>[2x]SETSRTAFGGRRAVPPNNSNAAEDDLPTVELQGVVPRGVNLQEFLNVTSVHLFKERWDTNKVDHHTDKYENNKLIVRRGQSFYVQIDFSRPYDPRRDLFRVEYVIGRYPQENKGTYIPVPIVSELQSGKWGAKIVMREDRSVRLSIQSSPKCIVGKFRMYVAV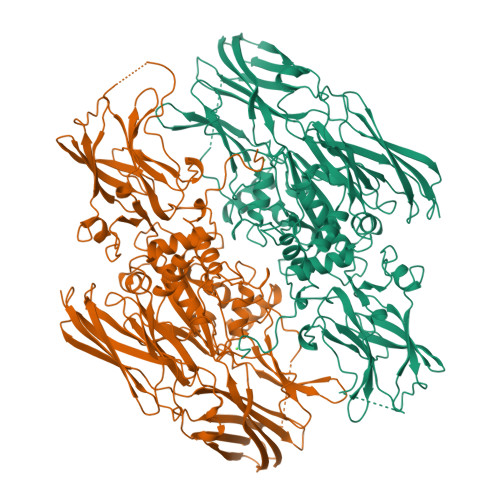WTPYGVLRTSRNPETDTYILFNPWCEDDAVYLDNEKEREEYVLNDIGVIFYGEVNDIKTRSWSYGQFEDGILDTCLYVMDRAQMDLSGRGNPIKVSRVGSAMVNAKDDEGVLVGSWDNIYAYGVPPSAWTGSVDILLEYRSSENPVRYGQCWVFAGVFNTFLRCLGIPARIVTNYFSAHDNDANLQMDIFLEEDGNVNSKLTKDSVWNYHCWNEAWMTRPDLPVGFGGWQAVDSTPQENSDGMYRCGPASVQAIKHGHVCFQFDAPFVFAEVNSDLIYITAKKDGTHVVENVDATHIGKLIVTKQIGGDGMMDITDTYKFQEGQEEERLALETALMYGAKKPLNTEGVMKSRSNVDMDFEVENAVLGKDFKLSITFRNNSHNRYTITAYLSANITFYTGVPKAEFKKETFDVTLEPLSFKKEAVLIQAGEYMGQLLEQASLHFFVTARINETRDVLAKQKSTVLTIPEIIIKVRGTQVVGSDMTVTVEFTNPLKETLRNVWVHLDGPGVTRPMKKMFREIRPNSTVQWEEVCRPWVSGHRKLIASMSSDSLRHVYGELDVQIQRRPSM>MTSSLHPTRGKLLKRFAQIGPYIREQQCQESQFFFDCLAVCVNKKVTPEKREFWGWWMELERNGEQLIYYYQVGLFDKNGDWVNQVISKKDVIESIHETLIRFHDFLQAAVSELEMTLVPDEKMSNFPLPL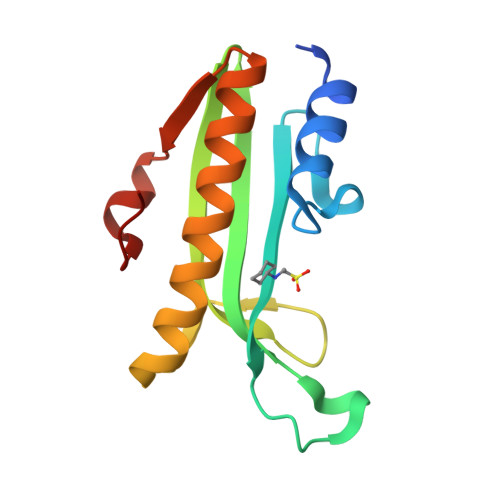KP[2x]> MAIATYNSHVELAKYLVSKADSVYLTIGKSTPWSNETNPPQPDENATVLQEVIGYKKATKVTLVRPSKSPEDDNKNLISYGNKSWVEVTPENAKAEGAKWVYLESSIVGDELPLGTYRQVGFV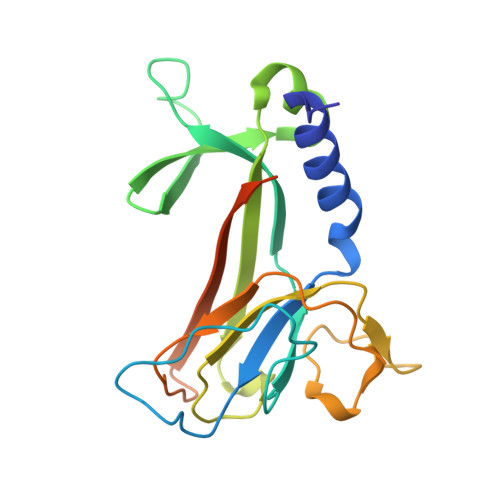MDLVAKSGISKFNLVPSEVESTGTLLFFDNKQFQNRSEQTTAKERFIVEVDPNSSSVDKLAAALEHHHHHH>[2x]FQHMGTVSWNLREMLAHAEETRKLMPVCVETKAIVSTIQRKYKGIKIQEGVVDYGARFYFYTSKTTVASLINTLNDLNETLVTMPLGYVTHGLNLEEAARYMRSLKVPATVSVSSPDA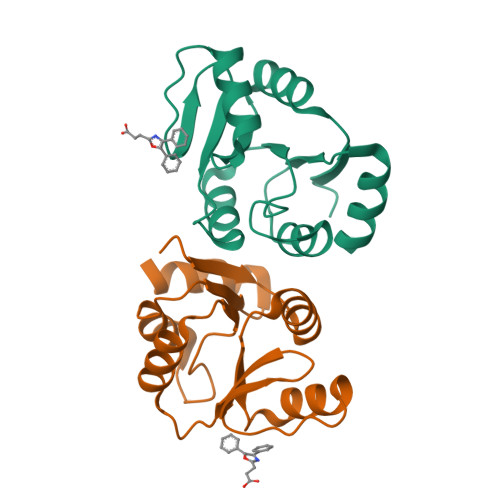VTAYNGYLTSS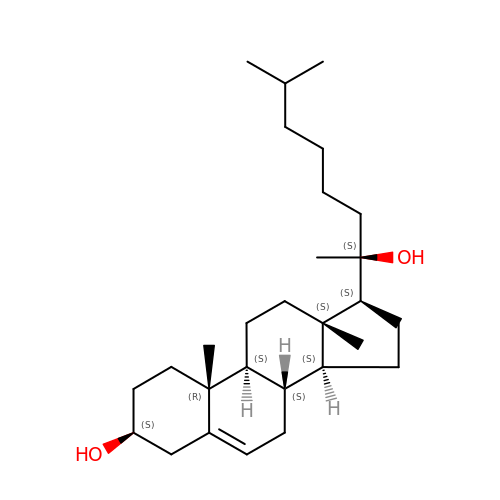20alpha-hydroxy-20-(5-methylhexyl)cholesterol | C28 H48 O2 | SVUJFWOKISPNOQ-VXBMVYAYSA-N> SGLEVLFQGPRSDAERGVCACPRI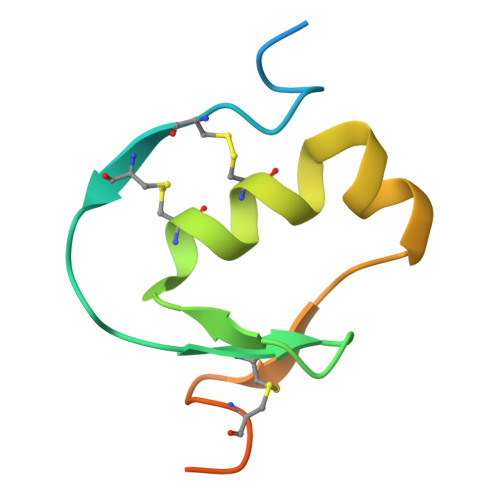YMPVCGSNLKTYNNDCLLRCEINSDLGRANNLRKIADQACDNLTDNVNDFIPQEY>QFPRQCATVEALRSGMCCPDLSPVSGPGTDRCGSSSGRGRCEAVTADSRPHSPQYPHDGRDDREVWPLRFFNRTCHCNGNFSGHNCGTCRPGWRGAACDQRVLIVRRNLLDLSKEEKNHFVRALDMAKRTTHPLFVIATRRSEEILGPDGNTPQFENISIYNYFVWTHYYSVKKTFLGVGQESFGEVDFSHEGPAFLTWHRYHLLRLEKDMQEMLQEPSFSLPYWNFATGKNVCDICTDDLMGSRSNFDSTLISPNSVFSQWRVVCDSLEDYDTLGTLCNSTEDGPIRRNPAGNVARPMVQRLPEPQDVAQCLEVGLFDTPPFYSNSTNSFRNTVEGYSDPTGKYDPAVRSLHNLAHLFLNGTGGQTHLSPNDPIFVLLHTFTDAVFDEWLRRYNADISTFPLENAPIGHNRQYNMVPFWPPVTNTEMFVTA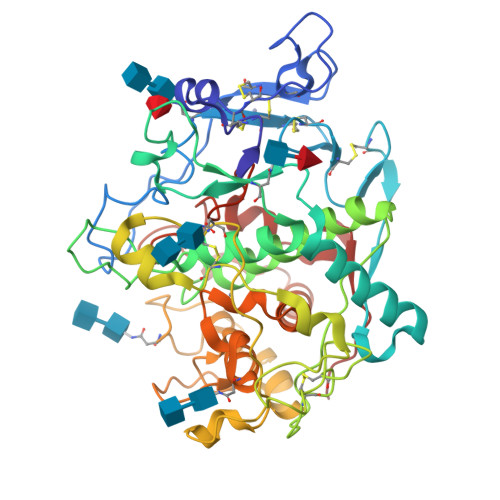PDNLGYTYEIQWPS[4x]>MIPEFSSFVVRTNTCGELRSSHLGQEVTLCGWIQYRRQNTFLVLRDFDGLVQVIIPQDESAASVKKILCEAPVESVVQVSGTVISRPAGQENPKMPTGEIEIKVKTAELLNACKKLPFEIKNFVKKTEALRLQYRYLDLRSFQMQYNLRLRSQMVMKMREYLCNLHGFVDIETPTLFKRTPGGAKEFLVPSREPGKFYSLPQSPQQFKQLLMVGGLDRYFQVARCYRDEGSRPDRQPEFTQIDIEMSFVDQTGIQSLIEGLLQYSWPNDKDPVVVPFPTMTFAEVLATYGTDKPDTRFGMKIIDISDVFRNTEIGFLQDALSKPHGTVKAICIPEGAKYLKRKDIESIRNFAADHFNQEIL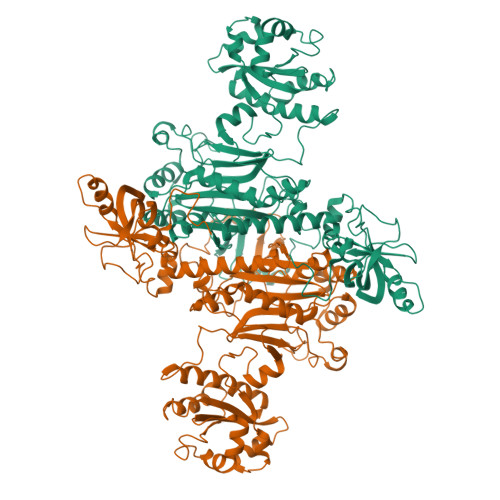PVFLNANRNWNSPVANFIMESQRLELIRLMETQEEDVVLLTAGEHNKACSLLGKLRLECADLLETRGVVLRDPTLFSFLWVVDFPLFLPKEENPRELESAHHPFTAPHPSDIHLLYTEPKKARSQHYDLVLNGNEIGGGSIRIHNAELQRYILATLLKEDVKMLSHLLQALDYGAPPHGGIALGLDRLICLVTGSPSIRDVIAFPKSFRGHDLMSNTPDSVPPEELKPYHIRVSKPTDSKAERAHVMYLEHHHHHH[4x]> GPGSCPTHADSLNNLANIKREQGNIEEAVRLYRKALEVFPEFAAAHSNLASVLQQQGKLQEALMHYKEAIRISPTFADAYSNMGNTLKEMQDVQGALQCYTRAIQINPAFADAHSNLASIHKDSGNIPEAIASYRTALKLKPDFPDAYCNLAHCLQIVCDWTDYDERMKKLVSIVADQLEKNRLPSVHPHHSMLYPLSHGFRKAIAERHGNLCLDKINVLHKPPYEHPKDLKLSDGRLRVGYVSSDFGNHPTSHLMQSIPGMHNPDKFEVFCYALSPDDGTNFRVKVMAEANHFIDLSQIPCNGKAADRIHQDGIHILVNMNG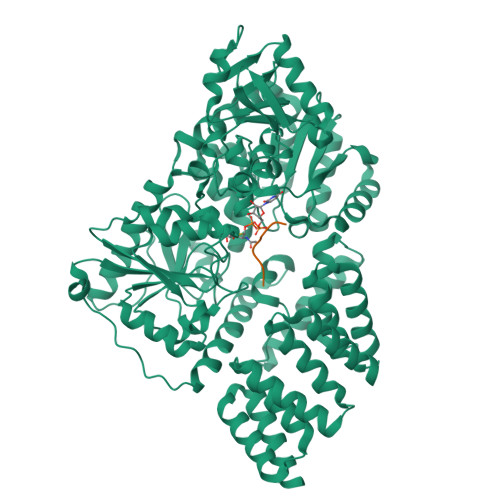YTKGARNELFALRPAPIQAMWLGYPGTSGALFMDYIITDQETSPAEVAEQYSEKLAYMPHTFFIGDHANMFPHLKKKAVIDFKSNGHIYDNRIVLNGIDLKAFLDSLPDVKIVKMKCPDGGDNADSSNTALNMPVIPMNTIAEAVIEMINRGQIQITINGFSISNGLATTQINNKAATGEEVPRTIIVTTRSQYGLPEDAIVYCNFNQLYKIDPSTLQMWANILKRVPNSVLWLLRFPAVGEPNIQQYAQNMGLPQNRIIFSPVAPKEEHVRRGQLADVCLDTPLCNGHTTGMDVLWAGTPMVTMPGETLASRVAASQLTCLGCLELIAKNRQEYEDIAVKLGTDLEYLKKVRGKVWKQRISSPLFNTKQYTMELERLYLQMWEHYAAGNKPDHMIKPVE;> KLSPSPSSRVTVS> QDSTSDLIPAPPLSKVPLQQNFQDNQFHGKWYVVGFAGNAILREDKDPQKMFATIYELKEDKSYNVTSVLFRKKK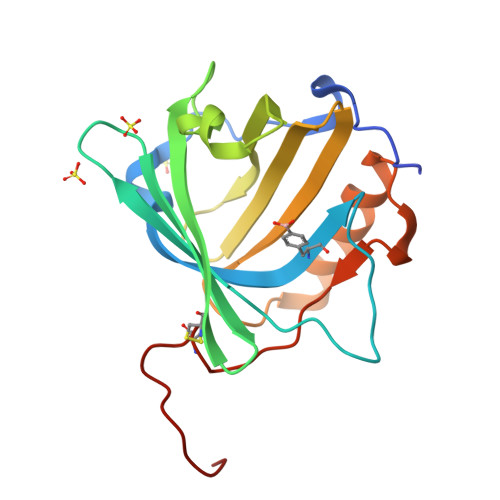CDYWIRTFVPGSQPGEFTLGNIKSYPGLTSYLVRVVSTNYNQHAMVFFKWVSQNREYFNITLYGRTKELTSELKENFIRFSKSLGLPENHIVFPVPIDQCIDGSAWSHPQFEK> GSASDIAQFLTDSGMKAIEDCSWNPIMQ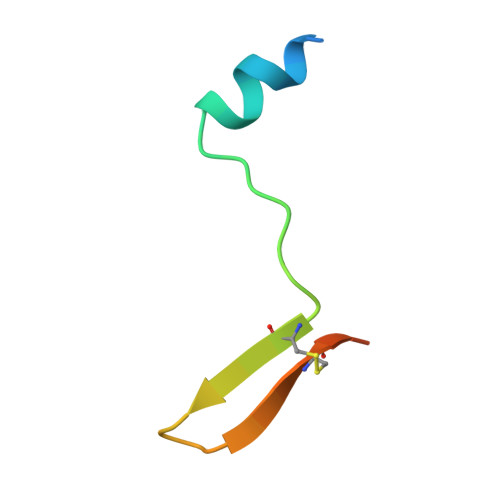QMACVVVAGSGS> GDVVATKLDPSRDLVRQKSRGRKNQMRSLVGRSNQHITHQSRPYTNEYASPCQITPPQEIKAPKENVWYGLTDDETADVAKWLFGRPELNLTTTENAGEWDNTIALIELHRPNKSEAIPYLDGSGPAPTRHAHVRLNNRATTDPYFADILVGPLPVSNATTWEPLEFPYTRKTQGQVRNVEPDGETVYSEWLFKISASIADITLDLWNGTALGLENDTLDIWGIDPLWQDDGRIIRWDMFWNMADDEFDSETLLPLGLYLKS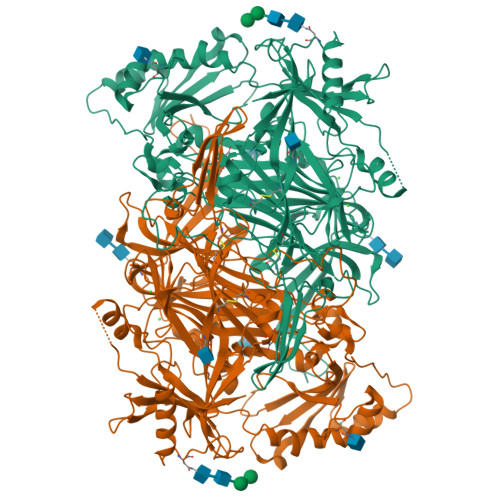DVTGRDPSQWKLLGWMYNDIFYETTEEFRKAYWSPGFVKLKPNVDGAWAHTEQRGPVPPQDRKQPPVMIAPDGARYSVDAERKYVTWMDFSFYIAFNRDTGLSLFDIKYKGQRVLYELGLQEALAHYAANDPVQSSVAYLDSYYGFGPYAFELLKGYDCPSYASYLNTSFYKDEETHTHVDSLCLFEFDADYPMARHSTSEFVSVTKNVYFTLRSVSTIGNYDYMFSYNFHMDGTIGVEVRASGYIQSAYYANNQDFGYQIHDSLSGSMHDHVLNFKADFDILGPNNTIELVSVVPVTKQFSWSGNKTRNTMQLGRSFIHSEDEARLNWGFNGQTQLHVVNQDKPNKFGEPRGYRILPSAGTAHLTVLNSSNLVHAAHWAEYDVQVTRQHDFEPTSAHPYNSQDIHNPPVDFSTFFNGESLNQTDLVVWLNLGMHHVPHTGDLPNTVFTTAHSGVAFTPLNYLPGDPSRETVNMVRVDYSDGAATAVRTFGQSNETCSVVLQPVENELWSYQGDVVVRKFPYDPNDPFYETDSDA>[2x]MSKTNVRIGAFEIDDAELHGEHQGERTLS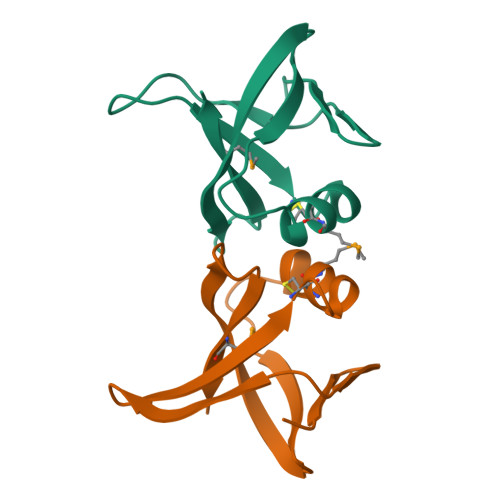IPCKSDPDLCMQLDAWDADTSVPAILNGEHSVLYRKHYDRQSDAWVMRLA> GMEAKLSSIEIPVGQDELSGTLLTPTGMP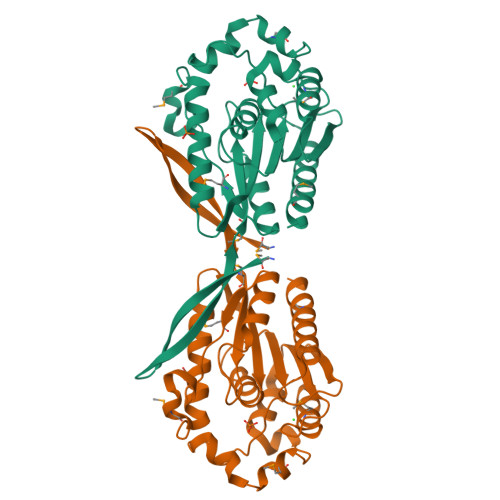GVLFVHGWGGSQHHSLVRAREAVGLGCICMTFDLRGHEGYASMRQSVTRAQNLDDIKAAYDQLASLPYVDAHSIAVVGLSYGGYLSALLTRERPVEWLALRSPALYKDAHWDQPKVSLNADPDLMDYRRRALAPGDNLALAACAQYKGDVLLVEAENDVIVPHPVMRNYADAFTNARSLTSRVIAGADHALSVKEHQQEYTRALIDWLTEMVVGRRIALAKEVVAARKQLLKEQQGDAVSLPGQGSREFRGDIRAVEKTSA> MQVNRLPFFTNHFFDTYLLISEDTPVGSSVTQLLARDMDNDPLVFGVSGEEASRFFAVEPDTGVVWLRQPLDRETKSEFTVEFSVSDHQGVITRKVNIQVGGVNDNAPTFHNQPYSVRIPENTPVGTPIFIVNATDPDLGAGGSVLYSFQPPSPFFAIDSARGIVTVIQELDYEVTQAYQLTVNATDQDKTRPLSTLANLAIIITDLEHHHHHH;> MQYDDDWQYEDCKLARGGPPATIVAIDEESRNGTILVDNMLIKGTAGGPDPTIELSLKDNVDYWVLLDPVKQMLFLNSTGRVLDRDPPMNIHSIVVQVQCVNKKVGTVIYHEVRIVVRDRNDNSPTFKHESYYATVNELTPVGTTIFTGFSGDNGATDIDDGPNGQIEYVIQYNPEDPTSNDTFEIPLML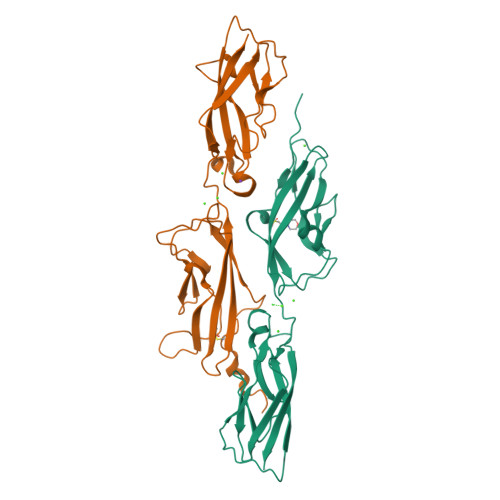TGNVVLRKRLNYEDKTRYYVIIQANDRAQNLNERRTTTTTLTVDLEHHHHHH>MAEAGITGTWYNQLGSTFIVTAGADGALTGTYESAVGNAESRYVLTGRYDSAPATDGSGTALG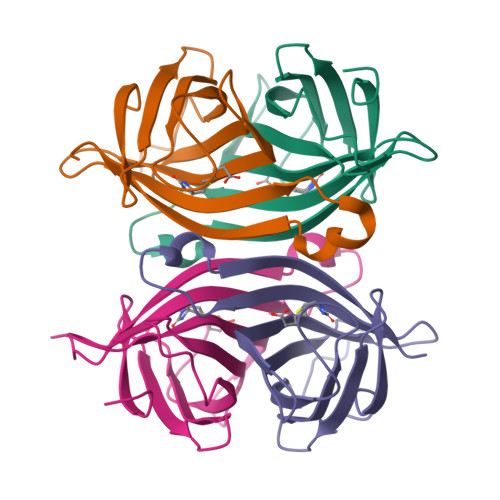WTVAWKNNYRNAHSATTWSGQYVGGAEARINTQWLXTSGTTEANAWKSTLVGHDTFTKVKPSAASLEHHHHHH[4x]>MGSSHHHHHHQNVSLQPPPQQLIVQNKTIDLPAVYQLNGGEEANPHAVKVLKELLSGKQSSKKGMLISIGEKGDKSVRKYSRQIPDHKEGYYLSVNEKEIVLAGNDERGTYYALQTFAQLLKDGKLPEVEIKDYPSVRYRGVVEGFYGTPWSHQARLSQLKFYGKNKMNTYIYGPKDDPYHSAPNWRLPYPDKEAAQLQELVAVANENEVDFVWAIHPGQDIKWNKEDRDLLLAKFEKMYQLGVRSFAVFFDDISGEGTNPQKQAELLNYIDEKFAQVKPDINQLVMCPTEYNKSWSNPNGNYLTTLGDKLNPSIQIMWTGDRVISDITRDGISWINERIKRPAYIWWNFPVSDYVRDHLLLGPVYGNDTTIAKEMSGFVTNPMEHAESSKIAIYSVASYAWNPAKYDTWQTWKDAIRTILPSAAEELECFAMHNSDLGPNGHGYRREESMDIQPAAERFLKAFKEGKNYDKADFETLQYTFERMKESADILLMNTENKPLIVEITPWVHQFKLTAEMGEEVLKMVEGRNESYFLRKYNHVKALQQQMFYIDQTSNQNPYQPGVKTATRVIKPLIDRTFATVVKFFNQKFNAHLDATTDYMPHKMISNVEQIKNLPLQVKANRVLISPANEVVKWAAGNSVEIELDAIYPGENIQINFGKDAPCTWGRLEISTDGKEWK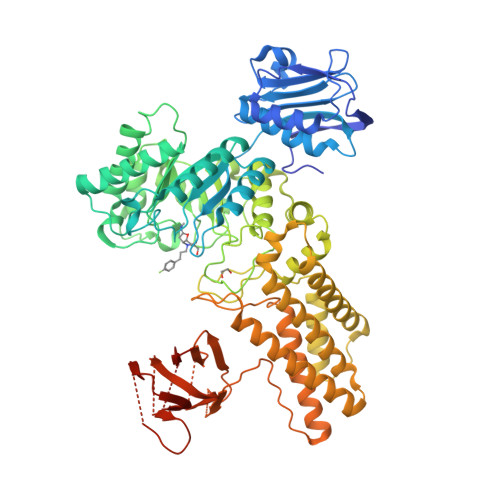TVDLKQKESRLSAGLQKAPVKFVRFTNVSDEEQQVYLRQFVLTIEKK[2x]>MADLAESNIKVMCRFRPLNESEVNRGDKYIAKFQGEDTVVIASKPYAFDRVFQSSTSQEQVYNDAAKKIVKDVLEGYNGTIFAYGQTSSGKVHTMEGKLHDPEGMGIIPRIVQDIFNYIYSMDENLEFHIKVSYFEIYLDKIRDLLDVSKTNLSVHEDKNRVPYVKGATERFVSSPDEVMDTIDEGKSNRHVAVTNMNEHSSRSHSIFLINVKQENTQTEQKLSGKLYLVDLAGSEKVSKTGAEGAVLDEAKNINKSLSALGNVISALAEGSTYVPY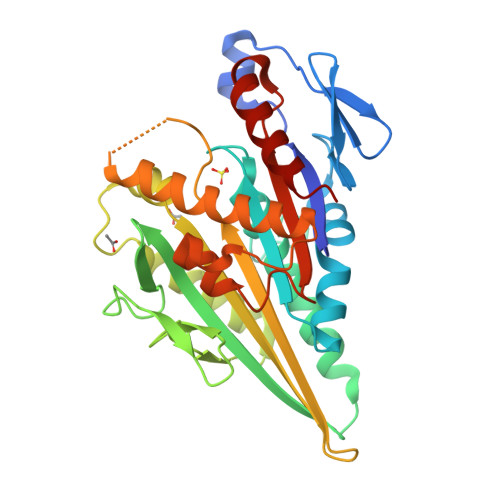RDSKMTRILQDSLGGNARTTIVICCSPSSYNESETKSTLLFGQRAKTI[2x]>[5x]EAEAYVEFDRADILYNIRQTSRPDVIPTQRDRPVAVSVSLKFINILEVNEITNEVDVVFWQQTTWSDRTLAWNSSHSPD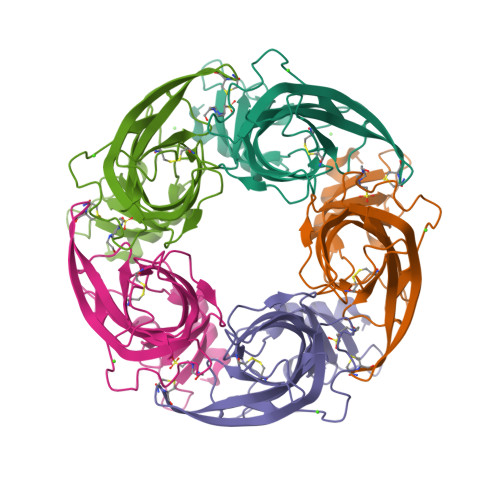QVSVPISSLWVPDLAAYNAISKPEVLTPQLARVVSDGEVLYMPSIRQRFSCDVSGVDTESGATCRIKIGSWTHHSREISVDPTTENSDDSEYFSQYSRFEILDVTQKKNSVTYSCCPEAYEDVEVSLNFRKKGRSEIL> GSMGSQTVDLSCLSGTTVRFFGPSHHFGGFTPLYDPAPDKRVATVDAGANALFIGGGGLNGQFAKTLLEEAEKHGIRLTPEELSQHSQ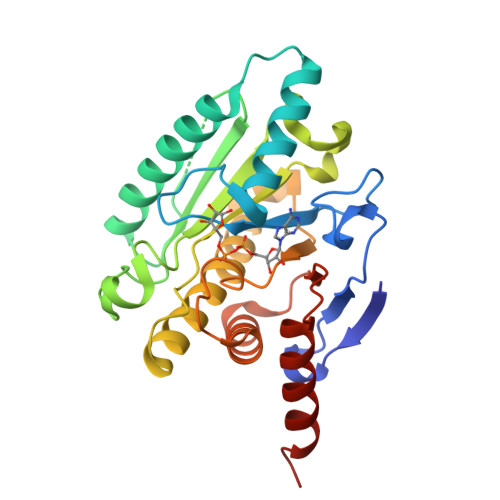RIQQSLLRRAVKSPGKLVELDTGVASPVFARSFGFVPVVPGLMWEESEVGPNVGVTFVHILKPEVTPYGNLNNNVMMYTVAPSGAAPDKTYSLAYKTTIAGVIGAAAAYNDTPAGQQYPVQGLRLPLLGGGIFRRNRSLESIGRANAEGTSLAITRYGPNFELQYMYDPSNAALHGLQEAESTYLASAAA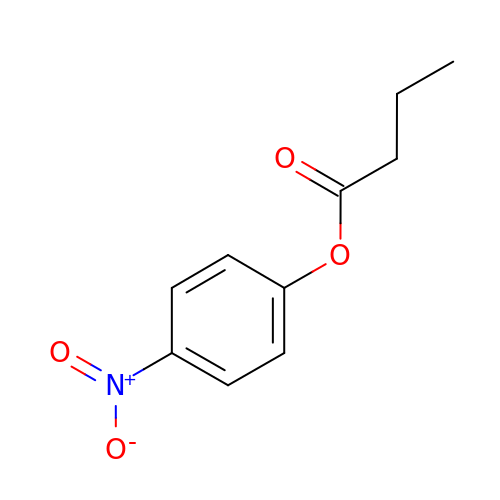(4-nitrophenyl) butanoate | C10 H11 N O4 | DVDUMIQZEUTAGK-UHFFFAOYSA-N>[4x]KPRKARTAFSDHQLNQLERSFERQKYLSVQDRMDLAAALNLTDTQVKTWYQNRRTKWKRQTA

Transcription factors (TFs) recognize specific bases within their DNA-binding motifs, with each base contributing nearly independently to total binding energy. However, the energetic contributions of particular dinucleotides can deviate strongly from the additive approximation, indicating that some TFs can specifically recognize DNA dinucleotides. Here we solved high-resolution (<1 Å) structures of MYF5 and BARHL2 bound to DNAs containing sets of dinucleotides that have different affinities to the proteins. The dinucleotides were recognized either enthalpically, by an extensive water network that connects the adjacent bases to the TF, or entropically, by a hydrophobic patch that maintained interfacial water mobility.

Another sequence, DNATC is also only one Hamming distance away from both local optima but has an even weaker affinity to BARHL2 than DNAAT. The recognition pattern appears to be a mixture of DNATT and DNAAC, with the hydrophobic contact of DNATT between C7 of T7 and the methyl group of Thr278 retained but at a sub-optimal distance (4.3 Å). The water molecules are arranged near Asn282 in a somewhat similar pattern to those observed in DNAAC, with the water net connecting the side-chain oxygens of Thr285 and Asn282 and N7 and O6 of G17 (opposite to C of AC). Thus, DNATC combines aspects of recognition from DNATT and DNAAC, but both types of interactions are less optimal, explaining the relatively low affinity of the BARHL2–DNATC complex.(2E)-3-[4-HYDROXY-3-(5,5,8,8-TETRAMETHYL-3-PROPOXY-5,6,7,8-TETRAHYDRONAPHTHALEN-2-YL)PHENYL]ACRYLIC 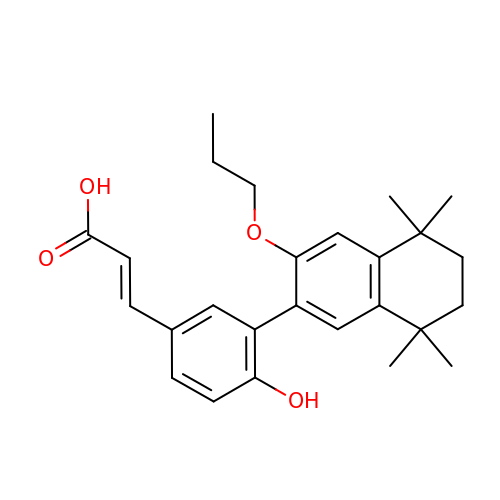ACID | C26 H32 O4 | DJVKZKGDIQNPRJ-CSKARUKUSA-N> SPSAEECGYSDRVRS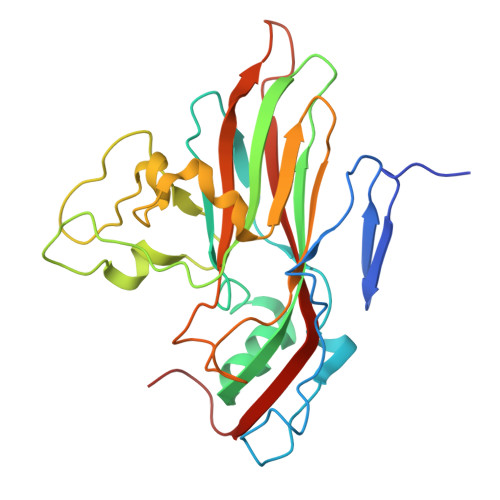ITLGNSTITTQECANVVVGYGVWPAYLKDEEATAEDQPTQPDVATCRFYTLESVMWQQGSPGWWWKFPDALSNMGLFGQNMQYHYLGRAGYTIHVQCNASKFHQGCLLVVCVPEAEMGCATLANKPDPKSLSKGEIASTFESQNSTGETAVQANVINAGMGVGVGNLTIFPHQWINLRTNNSATIVMPYINSVPMDNMFRHNNFTLMVIPFAPLSYSAGATTYVPITVTVAPMCAEYNGLRLAGKQ> MTIAERLRQEGEQSKALHIAKIMLESGVPLA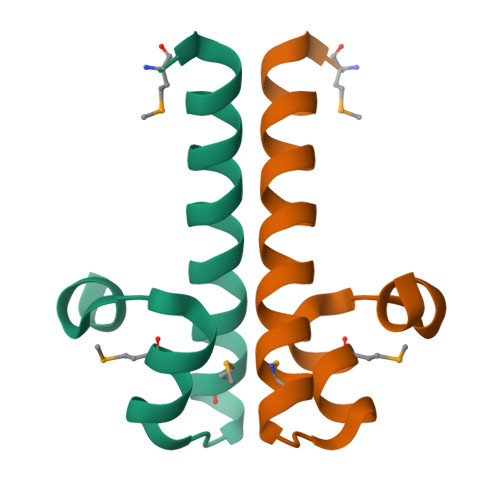DIMRFTGLSEEELAAASQ> MTDQPDLFGLAPDAPRPIIPANLPEDWQEALLPEFSAPYFHELTDFLRQERKEYTIYPPAPDVFNALRYTPLGEVKVLILGQDPYHGPNQAHGLSFSVRPGVRVPPSLRNIYKELTEDIPGFVAPKHGYLRSWAEQGVLLLNAVLTVRAGQANSHQGKGWEHFTDAVIKAVNAK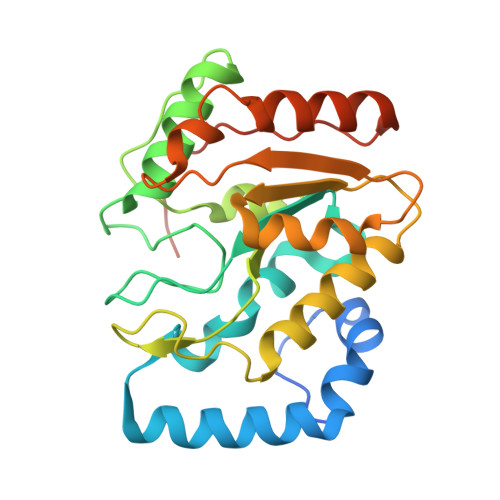EERVVFILWGSYARKKKKLITGKNHVVIESGHPSPLSEQYFFGTRPFSKTNEALEKAGRGPVEWQLPATVTEELEHHHHHH>GMTQHLTIAQTYLAAWNEEDNERRRHLVGQAWAENTRYVDPLMQGEGQQGIAAMIEAARQKFPGYR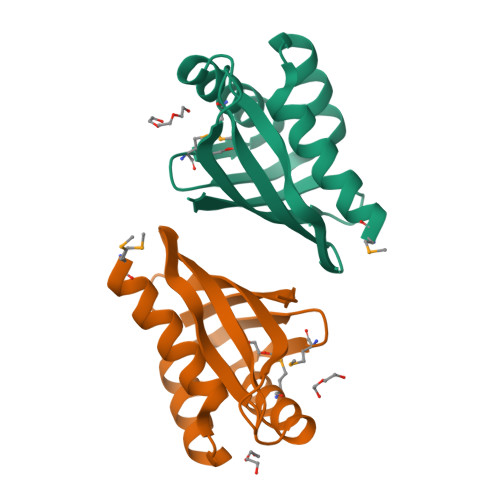FVLAGTPDGHGNFTRFSWRLISPDGDDVAGGTDVVSLNTEGRIDNVVGFLDGAVS[2x]> MGSSHHHHHHSQDPMNILLVSQCEKRALSETRRILDQFAERRGERTWQTPITQAGLDTLRRLLKKSARRNTAVACHWIRGRDHSELLWIVGDASRFNAQGAVPTNRTCRDILRKEDENDWHSAEDIRLLTVMAALFHDIGKASQAFQAKLRNRGKPMADAYRHEWVSLRLFEAFVGPGSSDEDWLRRLADKRETGDAWLSQLARDDRQSAPPGPFQKSRLPPLAQAVGWLIVSHHRLPNGDHRGSASLARLPAPIQSQWCGARDADAKEKAACWQFPHGLPFASAHWRARTALCAQSMLERPGLLARGPALLHDSYVMHVSRLILMLADHHYSSLPADSRLGDPNFPLHANTDRDSGKLKQRLDEHLLGVALHSRKLAGTLPRLERQLPRLARHKGFTRRVEQPRFRWQDKAYDCAMACREQAMEHGFFGLNLASTGCGKT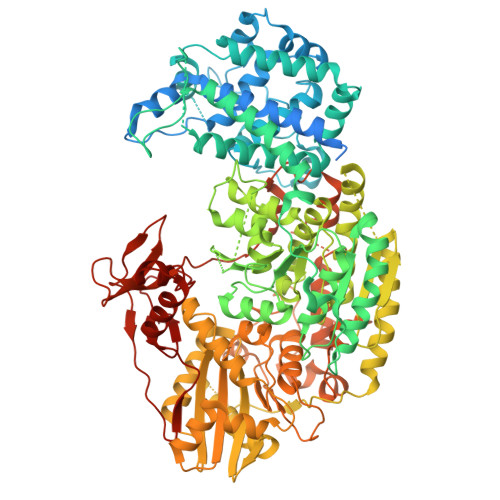LANGRILYALADPQRGARFSIALGLRSLTLQTGQAYRERLGLGDDDLAILVGGSAARELFEKQQERLERSGSESAQELLAENSHVHFAGTLEDGPLREWLGRNSAGNRLLQAPILACTIDHLMPASESLRGGHQIAPLLRLMTSDLVLDEVDDFDIDDLPALSRLVHWAGLFGSRVLLSSATLPPALVQGLFEAYRSGREIFQRHRGAPGRATEIRCAWFDEFSSQSSAHGAVTSFSEAHATFVAQRLAKLEQLPPRRQAQLCTVHAAGEARPALCRELAGQMNTWMADLHRCHHTEHQGRRISFGLLRLANIEPLIELAQAILAQGAPEGLHVHLCVYHSRHPLLVRSAIERQLDELLKRSDDDAAALFARPTLAKALQASTERDHLFVVLASPVAEVGRDHDYDWAIVEPSSMRSIIQLAGRIRRHRSGFSGEANLYLLSRNIRSLEGQNPAFQRPGFETPDFPLDSHDLHDLLDPALLARIDASPRIVEPFPLFPRSRLVDLEHRRLRALMLADDPPSSLLGVPLWWQTPASLSGALQTSQPFRAGAKERCYALLPDEDDEERLHFSRYEEGTWSNQDNLLRNLDLTYGPRIQTWGTVNYREELVAMAGREDLDLRQCAMRYGEVRLRENTQGWSYHPYLGFKKYN>MSLTQQITLIKDKILSDNYFTLHNITYDLTRKDGEVIRHKREVYDRGNGATILLYNTKKKTVVLIRQFRVATWVNGNESGQLIESCAGLLDNDEPEVCIRKEAIEETGYEVGEVRKLFELYMSPGGVTELIHFFIAEYSDNQRANAGGGVEDEDIEVLEL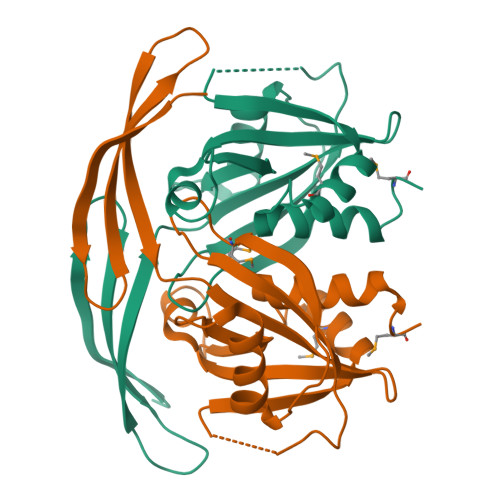PFSQALEMIKTGEIRDGKTVLLLNYLQTSHLMDEGGSHHHHHH[4x]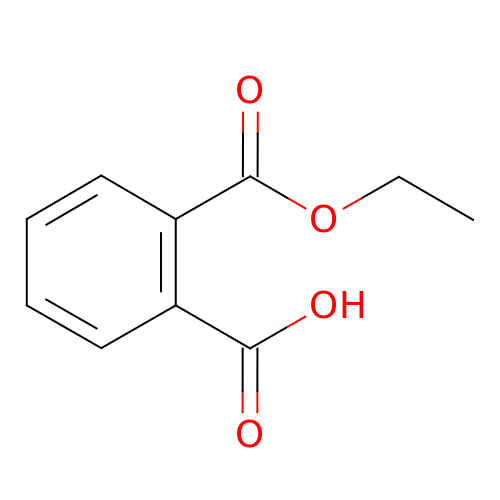2-ethoxycarbonylbenzoic acid | C10 H10 O4 | YWWHKOHZGJFMIE-UHFFFAOYSA-N>[4x]MHHHHHHARATGK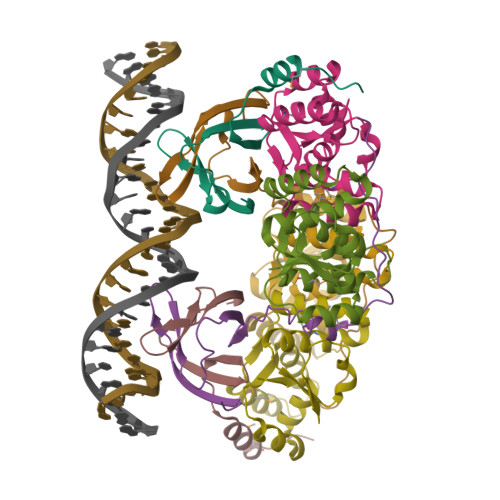TFRSGNSEAVRLPRDLAFGADVELTLIRSGDVLTIYPSKGSIADLVATLNQMPRPDSVEIRDEDLFPERPGL;>[4x]MAYVLDTNVAIHLRDGDPEVTTRVTALNGAILLSIISRVELEGGVYREAAQAGLRRSRLDVMLKVLPVLDFDGAAADEYRRIVESAGYSRRKVVDRMIAAQALAHRATFVTFNADDFRDIPGLSLLAW1,3-BUTANEDIOL 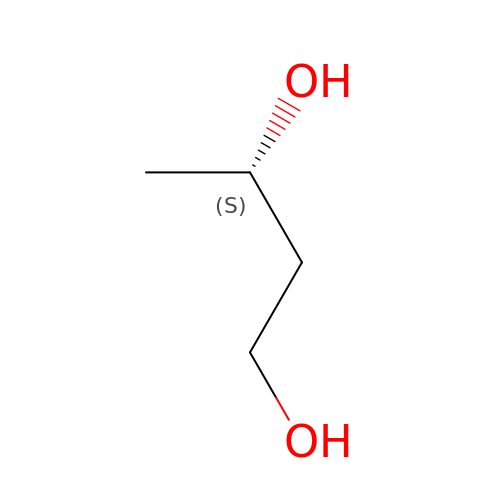| C4 H10 O2 | PUPZLCDOIYMWBV-BYPYZUCNSA-N[2,6-bis(3-methoxyphenyl)-1-benzofuran-3-yl]acetic 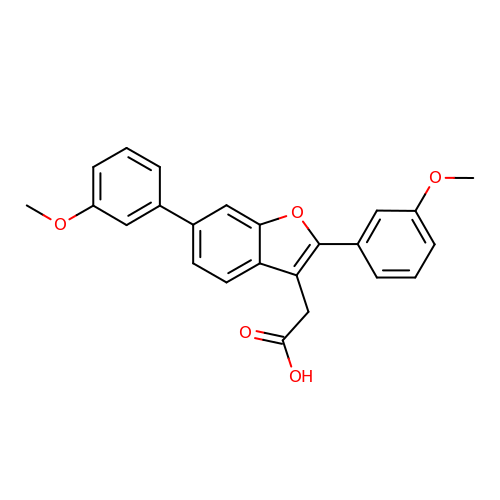acid | C24 H20 O5 | DPEJTEZYXSGVKK-UHFFFAOYSA-N>MSLDKGDKAPDFALPGKTGVVKLSDKTGS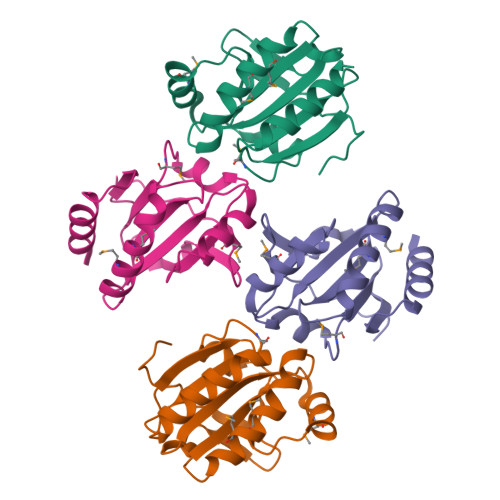VVYLDFWASWCGPCRQSFPWMNQMQAKYKAKGFQVVAVNLDAKTGDAMKFLAQVPAEFTVAFDPKGQTPRLYGVKGMPTSFLIDRNGKVLLQHVGFRPADKEALEQQILAALGGNEGHHHHHH[4x]>[2x]SRAKRIMKEIQAVKDDPAAHITLEFVSESDIHHLKGTFLGPPGTPYEGGKFVVDIEVPMEYPFKPPKMQFDTKVYHPNISSVTGAICLDILKNAWSPVITLKSALISL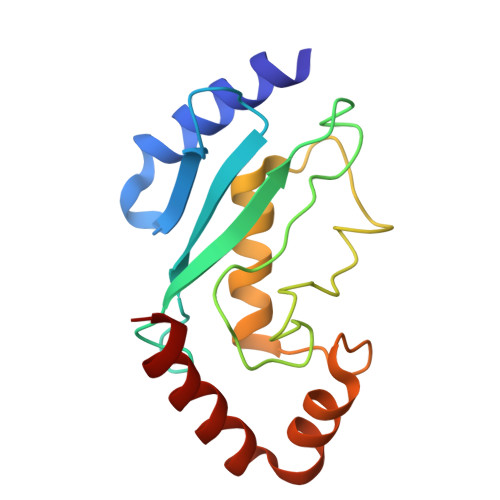QALLQSPEPNDPQDAEVAQHYLRDRESFNKTAALWTRLYAS>[2x]MSLRFALTPGEPAGIGPDLCLLLARSAQPHPLIAIASRTLLQERAGQLGLAIDLKDVSPAAWPERPAKAGQLYVWDTPLAAPVRPGQLDRANAAYVLETLTRAGQGCLDGHFAGMI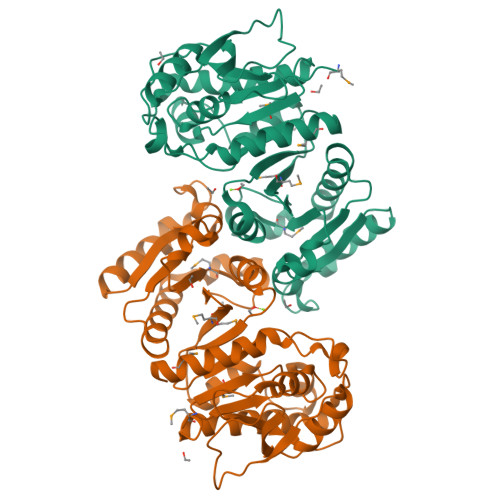TAPVHKGVINEAGIPFSGHTEFLADLTHTAQVVMMLATRGLRVALATTHLPLREVADAISDERLTRVARILHADLRDKFGIAHPRILVCGLNPHAGEGGHLGREEIEVIEPCLERLRGEGLDLIGPLPADTLFTPKHLEHCDAVLAMYHDQGLPVLKYKGFGAAVNVTLGLPIIRTSVDHGTALDLAGSGRIDSGSLQVALETAYQMAASRC>[4x]MKVGQDKVVTIRYTLQVEGEVLDQGELSYLHGHRN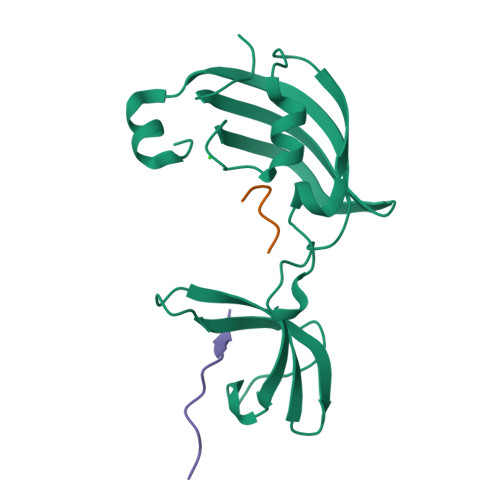LIPGLEEALEGREEGEAFQAHVPAEKAYGPHDPEGVQVVPLSAFPEDAEVVPGAQFYAQDMEGNPMPLTVVAVEGEEVTVDFNHPLAGKDLDFQVEVVKVREATPEELLHGHAHLVPK;>TRYANPKMKPFIFGAX[9x]(E)-N-[(5-carbamimidamido-2-hydroxyphenyl)methylidene]-L-alanine | C11 H14 N4 O3 | 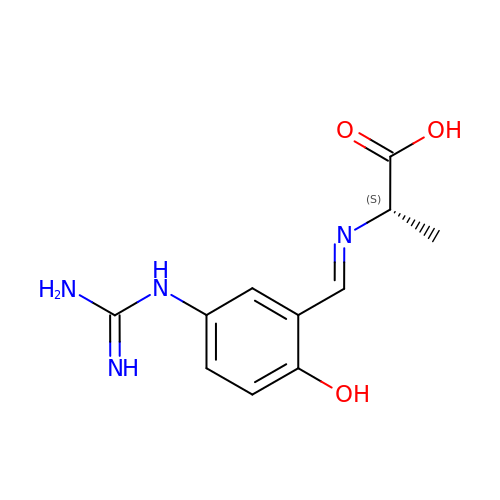XIDJFBOMDZEVTM-JHKKWMAKSA-N>MAHHHHHHMTCRTRFAPSPTGYLHIGGARTALYCWLEARHRGGEFVLRIEDTDRERSTQGAIDAILEAMEWLGLDYDEGPIYQTDRVARYLEVAEQLVADGKAYYAYETREELDAMREAAMARQEKPRYNGAARDLGLPRRDDPNRVIRFKNPLEGTVVFDDLIKGRIEIANSELDDMVIFRPDGYPTYNFAVVVDDWDMGITEVIRGDDHINNTPRQINLYEGIGAPVPKFGHMPMILDEQGAKLSKRTGAADVMQYKDAGYLPDALLSYLARLGWSHGDQELFSRQELIELFDVKDCNSKASRLDMAKLGWVNQHFLKTEDVAAIVPHLVYQLQKLGLDVAAGPAPEDVVVALRERVQTLKEMAEKAVVWYQPLTEYDEAAVAKHFKAGAEVALGKARELLAALPEWTA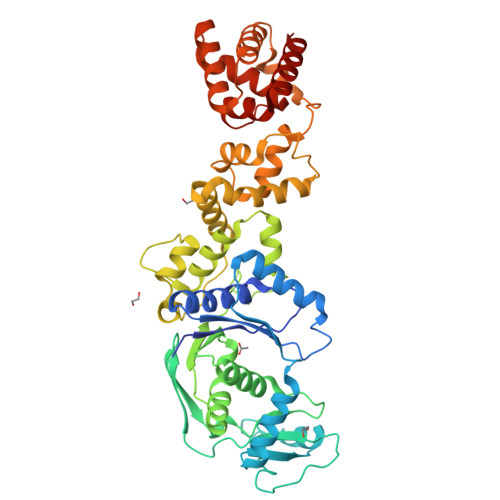ESVGVALHDAAAALEIGMGKVAQPLRVAITGTQVSPDISHTVYLAGREQALKRIDVAITKVATA[2x]>MRVLVGGGTGFIGTALTQLLNARGHE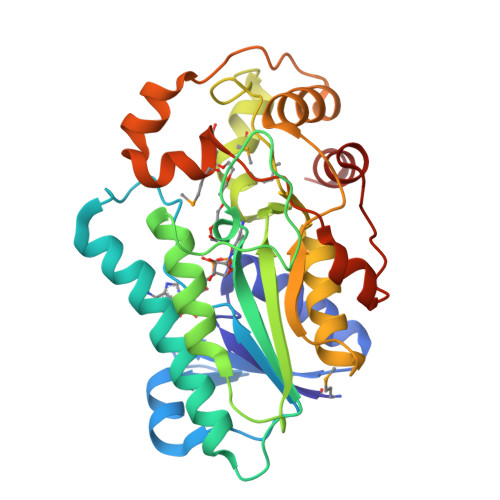VTLVSRKPGPGRITWDELAASGLPSCDAAVNLAGENILNPLRRWNETFQKEVLGSRLETTQLLAKAITKAPQPPKAWVLVTGVAYYQPSLTAEYDEDSPGGDFDFFSNLVTKWEAAARLPGDSTRQVVVRSGVVLGRGGGAMGHMLLPFRLGLGGPIGSGHQFFPWIHIGDLAGILTHALEANHVHGVLNGVAPSSATNAEFAQTFGAALGRRAFIPLPSAVVQAVFGRQRAIMLLEGQKVIPRRTLATGYQYSFPELGAALKEIAENLYFQ[8x]> DNGGYVPAVVIGTGYGAAVSALRLGEAGVQTLMLEMGQLWNQPGPDGNIFCGMLNPDKRSSWFKNRTEAPLGSFLWLDVVNRNIDPYAGVLDRVNYDQMSVYVGRGVGGGSLVNGGMAVEPKRSYFEEILPRVDSSEMYDRYFPRANSMLRVNHIDTKWFEDTEWYKFARVSREQAGKAGLGTVFVPNVYDFGYMQREAAGEVPKSALATEVIYGNNHGKQSLDKTYLAAALGTGKVTIQTLHQVKTIRQTKDGGYALTVEQKDTDGKLLATKEISCRYLFLGAGSLGSTELLVRARDTGTLPNLNSEVGAGW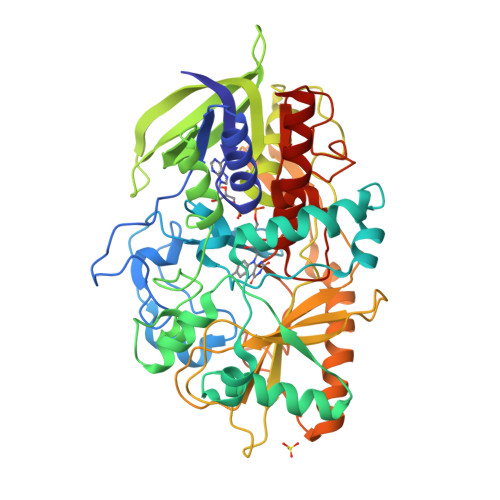GPNGNIMTARANHMWNPTGAHQSSIPALGIDAWDNSDSSVFAQIAPMPAGLETWVSLYLAITKNPQRGTFVYDAATDRAKLNWTRDQNAPAVNAAKALFDRINKANGTIYRYDLFGTQLKAFADDFCYQPLGGCVLGKATDDYGRVAGYKNLYVTDGSLIPGSVGVNPFVTITALAERNVERIIKQDVTAS> SDKIIHLTDDSFDTDVLKADGAILVDFWAEWCVWCKMIAPILDEIADEYQGKLTVAKLNIDQNPGTAPKYGIRGIPTLLLFKNGEVAA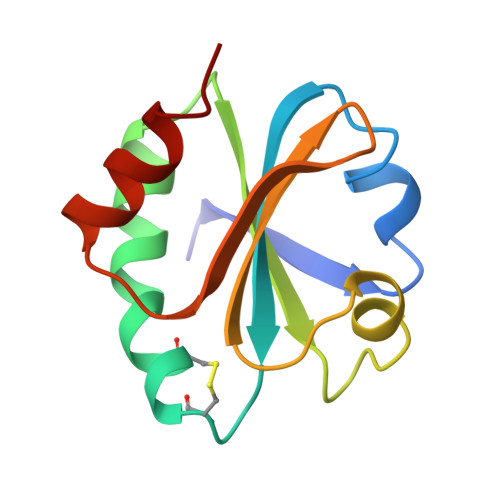TKVGALSKGQLKEFLDANLA>[2x]MHHHHHHMKYTVITGASSGIGYETAKLLAGKGKSLVLVARRTSELEKLRDEVKQISPDSDVILKSVDLADNQNVHDLYEGLKELDIETLINNAGFGDFDLVQDIELGKIEKMLRLNIEALTILSSLFARDHHDIEGTTLVNISSLGGYRIVPNAVTYCATKFYVSAYTEGLAQELQKGGAKLRAKVLAPAATETEFVDRARGEAGFDYSKNVHKYHTAAEMAGFLHQLIESDAIVGIVDGETYEFEL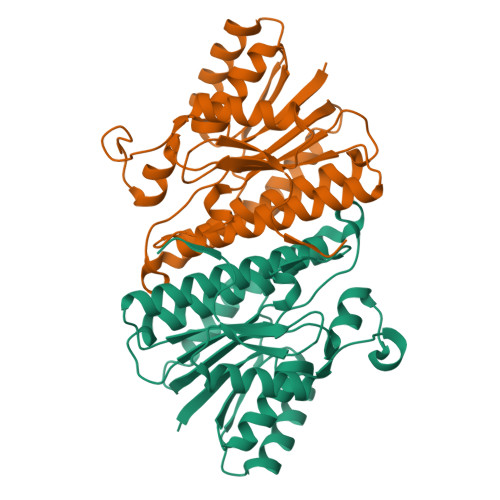RGPLFNYAG>[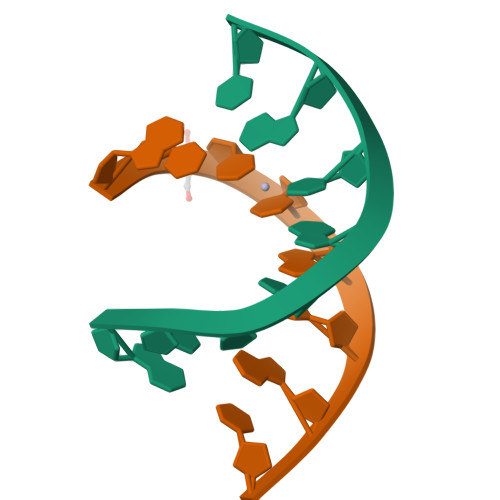2x]GCCCGTGC> GSHMVKEINESIFDEEIKT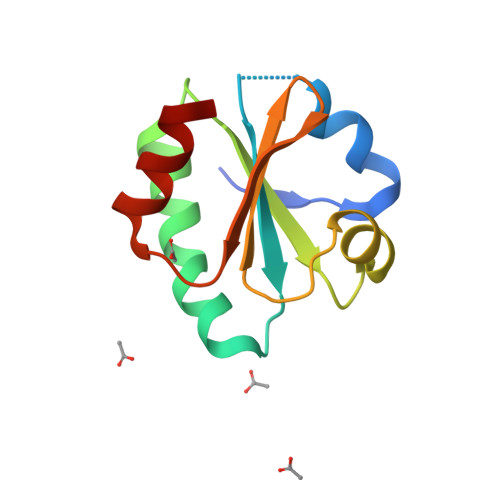SGEPVIVDFWAPWCGPCKMLGPIIDELSEDLDGKAKFTKVNVDENPGIASKFGIASIPTVMIFKDGNPVETLVGFRPKQSITASIEKHM> MENTENSVASKSIKNLEPKIIHGSESMASGISLDNSYKMDYPEMGL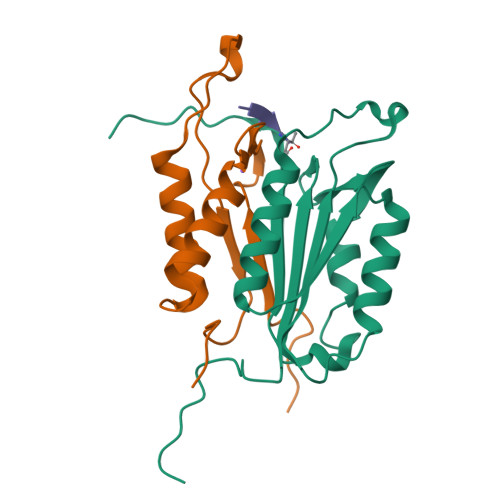CIIINNKNFHKSTGMTSRSGTDVDAANLRETFRNLKYEVRNKNDLTREEIVELMRDVSKEDHSKRSSFVCVLLSHGEEGIIFGTNGPVDLKKITNFFRGDRCRELTGKPKLFIIQACRGTELDCGIETD;> SGVDDDMACHKIPVEADFLYAYSTAPGYYSWRNSKDGSWFIQSLCAMLKQYADKLEFMHILTRVNRKVATEFESFSFDATFHAKKQIPCIVSMLTKELYFYHH> SVQQASRSKVSVAPLHLESAKEPPLNTYKPKEPFTATIVSVESLVGPKAPGETCHIVIDHGGNVPYWEGQSYGVIPPGENPKKPGAPQNVRLYSIASTRYGDNFDGRTGSLCVRRAVYYDPETGKEDPSKNGVCSNFLCNSKPGDKIQLTGPSGKIMLLPEEDPNATHIMIATGTGVAPFRGYLRRMFMEDVPNYRFGGLAWLFLGVANSDSLLYDEEFTS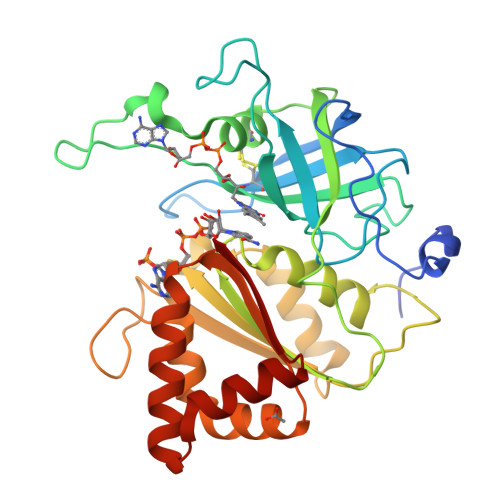YLKQYPDNFRYDKALSREQKNRSGGKMYVQDKIEEYSDEIFKLLDGGAHIYFCGLKGMMPGIQDTLKKVAERRGESWDQKLAQLKKNKQWHVEVS>VPRGSHMTDQAFVTLTTNDAYAKGALVLGSSLKQHRTSRRLAVLTTPQVSDTMRKALEIVFDEVITVDILDSGDSAHLTLMKRPELGVTLTKLHCWSLTQYSKCVFMDADTLVLANIDDLFEREELSAAPDPGWPDCFNSGVFVYQPSVETYNQLLHVASEQGSFDGGDQGLLNTFFNSWATTDIRKHLPFIYNLSSISIYSYLPAFKAFGANAKVVHFLGQTKPWNYTYDTKTKSVRSEGHDPTMTHPQFLNVWWDIFTTSVVPLLQQFGLVQDTCSYQHVEDVSGAVSHLSLGETPATTQPFVSSEERKERWEQG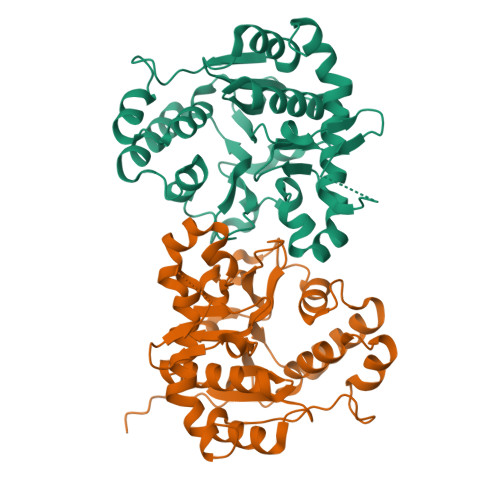QADYMGADSFDNIKKKLDTYLQ[10x]> MDNSHDSDSVFLYHIPCDNCGSSDGNSLFSDGHTFCYVCEKWTAGNEDTKERASKRKPSGGKPMTYNVWNFGESNGRYSALTARGISKETCQKAG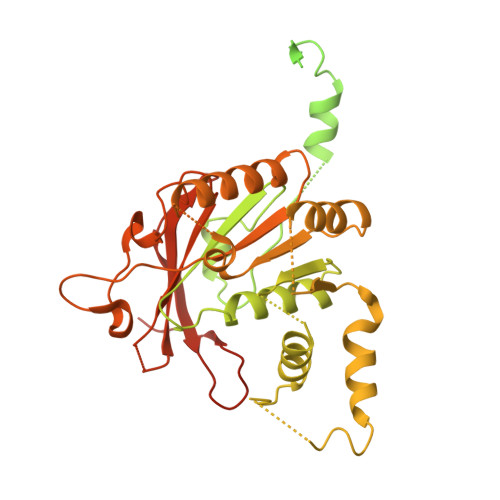YWIAKVDGVMYQVADYRDQNGNIVSQKVRDKDKNFKTTGSHKSDALFGKHLWNGGKKIVVTEGEIDMLTVMELQDCKYPVVSLGHGASAAKKTCAANYEYFDQFEQIILMFDMDEAGRKAVEEAAQVLPAGKVRVAVLPCKDANECHLNGHDREIMEQVWNAGPWIPDGVVSALSLRERIREHLSSEESVGLLFSGCTGINDKTLGARGGEVIMVTSGSGMGKSTFVRQQALQWGTAMGKKVGLAMLQESVEETAEDLIGLHNRVRLRQSDSLKREIIENGKFDQWFDELFGNDTFHLYDSFAEAETDRLLAKLAYMRSGLGCDVIILDHISIVVSASGESDERKMIDNLMTKLKGFAKSTGVVLVVICHLKNPDKGKAHEEGRPVSITDLRGSGALRQLSDTIIALERNQQGDMPNLVLVRILKCRFTGDTGIAGYMEYNKETGWLEPSSYSGEEESHSESTDWSNDTDF> MSGTFHGDGHAPMSPFEDTFQFEDNSSNEDTHIAPTHFDDGATSNKYSRPQVSFNDETPKNKREDAEEFTFNDDTEYDNHSFQPTPKLNNGSGTFDDVELDNDSGEPHTNYDGMKRFRMGTKRNKKGNPIMGRSKTLKWARKNIPNPFEDFTKDDIDPGAINRAQELRTVYYNMPLPKDMIDEEGNPIMQYPRNKIRTTKYTPLTFLPKNILFQFHNFANVYFLVLIILGAFQIFGVTNPGLSAVPLVVIVIITAIKDAIEDSRRTVLDLEVNNTKTHILEGVENENVSTDNISLWRRFKKANSRLLFKFIQYCKEHLTEEGKKKRMQRKRHELRVQKTVGTSGPRSSLDSIDSYRVSADYGRPSLDYDNLEQGAGEANIVDRSLPPRTDCKFAKNYWKGVKVGDIVRIHNNDEIPADIILLSTSDTDGACYVETKNLDGETNLKVRQSLKCTNTIRTSKDIARTKFWIESEGPHSNLYTYQGNMKWRNLADGEIRNEPITINNVLLRGCTLRNTKWAMGVVMFTGGDTKIMLNSGITPTKKSRISRELNFSVVINFVLLFILCFVSGIANGVYYDKKGRSRFSYEFGTIAGSAATNGFVSFWVAVILYQSLVPISLYISVEIIKTAQAAFIYGDVLLYNAKLDYPCTPKSWNISDDLGQVEYIFSDKTGTLTQNVMEFKKCTINGVSYGRAYTEALAGLRKRQGIDVETEGRREKAEIAKDRDTMIDELRALSGNSQFYPEEVTFVSKEFVRDLKGASGEVQQRCCEHFMLALALCHSVLVEANPDNPKKLDLKAQSPDEAALVATARDVGFSFVGKTKKGLIIEMQGIQKEFEILNILEFNSSRKRMSCIVKIPGLNPGDEPRALLICKGADSIIYSRLSRQSGSNSEAILEKTALHLEQYATEGLRTLCIAQRELSWSEYEKWNEKYDIAAASLANREDELEVVADSIERELILLGGTAIEDRLQDGVPDCIELLAEAGIKLWVLTGDKVETAINIGFSCNLLNNEMELLVIKTTGDDVKEFGSEPSEIVDAL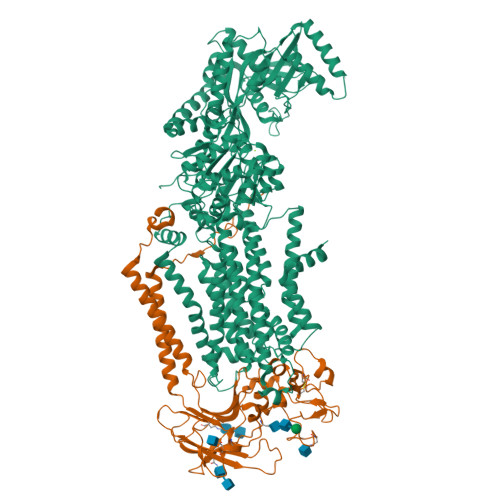LSKYLKEYFNLTGSEEEIFEAKKDHEFPKGNYAIVIDGDALKLALYGEDIRRKFLLLCKNCRAVLCCRVSPSQKAAVVKLVKDSLDVMTLAIGDGSNDVAMIQSADVGIGIAGEEGRQAVMCSDYAIGQFRYLARLVLVHGRWSYKRLAEMIPEFFYKNMIFALALFWYGIYNDFDGSYLYEYTYMMFYNLAFTSLPVIFLGILDQDVNDTISLVVPQLYRVGILRKEWNQRKFLWYMLDGLYQSIICFFFPYLVYHKNMIVTSNGLGLDHRYFVGVYVTTIAVISCNTYVLLHQYRWDWFSGLFIALSCLVVFAWTGIWSSAIASREFFKAAARIYGAPSFWAVFFVAVLFCLLPRFTYDSFQKFFYPTDVEIVREMWQHGHFDHYPPGYDPTDPNRPKVTKAGQHGEKIIEGIALSDNLGGSNYSRDSVVTEEIPMTFMHGEDGSPSGYQKQETWMTSPKETQDLLQSPQFQQAQTFGRGPSTNVRSSLDRTREQMIATNQLDNRYSVERARTSLDLPGVTNAASLIGTQQNN;> MVNFDLGQVGEVFRRKDKGAIVSGDNPEEEEDVDASEFEEDEVKPVRTKNRRPKEDAFTQQRLAAINPVLTPRTVLPLYLLIAVVFVIVGGCILAQNSKVDEVTIYYQDCMTNATSSWSDIPSEHWQFVFHKYKTYNTAPQWRFVDDESDDFTKQRGTCQIRFTTPSDMKNNVYLNYVLEKFAANHRRYVLSFSEDQIRGEDASYETVHDATGINCKPLSKNADGKIYYPCGLIANSMFNDTFPLQLTNVGDTSNNYSLTNKGINWESDKKRYKKTKYNYTQIAPPPYWEKMYPDGYNETNIPDIQDWEEFQNWMRPGAFDKITKLIRINKNDTLPAGEYQLDIGLHWPVLEFNGKKGIYLTHGSHLGGRNPFLGIVYLIGGCICAAMALILLTFWLFGGRKIADASSLSWNMK>SKEMQSCVDECLRCYQMCFGMAMTHCLETGGDHVKPKHFRAMISCAEMCRNAAHMMLMKSPQARHICEDCAEACEACAKECDALPDMKDCAAQCRRCAEAC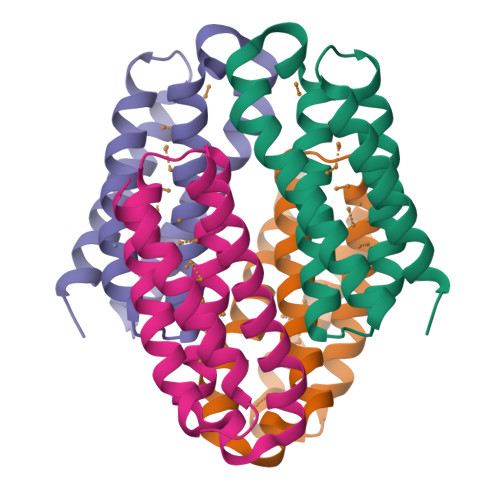RKMAGQK[4x]> MRGSHHHHHHGSELPQMVQQLNSPDQQELQSALRKLSQIASGGNEQIQAVIDAGALPALVQLLSSPNEQILQEALWALSNIASGGNEQIQAVIDAGALPALVQLLSSPNEQILQ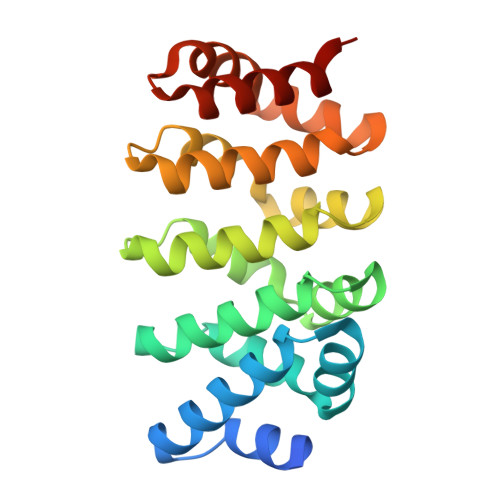EALWALSNIASGGNEQIQAVIDAGALPALVQLLSSPNEQILQEALWALSNIASGGNEQKQAVKEAGALEKLEQLQSHENEKIQKEAQEALEKLQSH> MEDVEIKPRGYQLRLVDHLTKSNGIVYLPTGSGKTFVAILVLKRFSQDFDKPIESGGKRALFMCNTVELARQQAMAVRRCTNFKVGFYVGEQGVDDWTRGMWSDEIKKNQVLVGTAQVFLDMVTQTYVALSSLSVVIIDECHHGTGHHPFREFMRLFTIANQTKLPRVVGLTGVLIKGNEITNVATKLKELEITYRGNIITVSDTKEMENVMLYATKPTEVMVSFPHQEQVLTVTRLISAEIEKFYVSLDLMNIGVQPIRRSKSLQCLRDPSKKSFVKQLFNDFLYQMKEYGIYAASIAIISLIVEFDIKRRQAETLSVKLMHRTALTLCEKIRHLLVQKLQDMTYDDDDDNVNTEEVIMNFSTPKVQRFLMSLKVSFADKDPKDICCLVFVERRYTCKCIYGLLLNYIQSTPELRNVLTPQFMVGRNNISPDFESVLERKWQKSAIQQFRDGNANLMICSSVLEEGIDVQACNHVFILDPVKTFNMYVQSKGRARTTEAKFVLFTADKEREKTIQQIYQYRKAHNDIAEYLKDRVLEKTEPELYEIKGHFQDDIDPFTNENGAVLLPNNALAILHRYCQTIPTDAFGFVIPWFHVLQEDERDRIFGVSAKGKHVISINMPVNCMLRDTIYSDPMDNVKTAKISAAFKACKVLYSLGELNERFVPKTLKERVASIADVHFEHWNKYGDSVTATVNKADKSKDRTYKTECPLEFYDALPRVGEICYAYEIFLEPQFESCEYTEHMYLNLQTPRNYAILLRNKLPRLA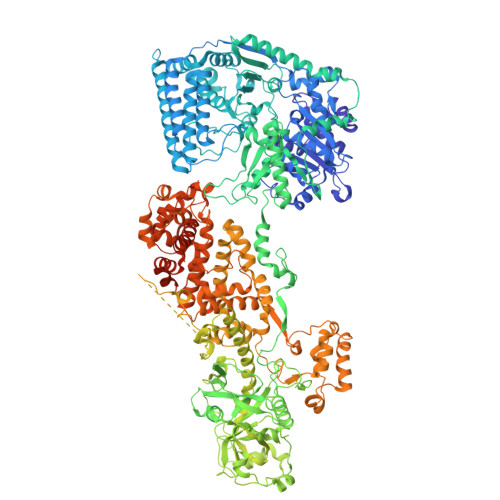EMPLFSNQGKLHVRVANAPLEVIIQNSEQLELLHQFHGMVFRDILKIWHPFFVLDRRSKENSYLVVPLILGAGEQKCFDWELMTNFRRLPQSHGSNVQQREQQPAPRPEDFEGKIVTQWYANYDKPMLVTKVHRELTPLSYMEKNQQDKTYYEFTMSKYGNRIGDVVHKDKFMIEVRDLTEQLTFYVHNRGKFNAKSKAKMKVILIPELCFNFNFPGDLWLKLIFLPSILNRMYFLLHAEALRKRFNTYLNLHLLPFNGTDYMPRPLEIDYSLKRNVDPLGNVIPTEDIEEPKSLLEPMPTKSIEASVANLEITEFENPWQKYMEPVDLSRNLLSTYPVELDYYYHFSVGNVCEMNEMDFEDKEYWAKNQFHMPTGNIYGNRTPAKTNANVPALMPSKPTVRGKVKPLLILQKTVSKEHITPAEQGEFLAAITASSAADVFDMERLEILGDSFLKLSATLYLASKYSDWNEGTLTEVKSKLVSNRNLLFCLIDADIPKTLNTIQFTPRYTWLPPGISLPHNVLALWRENPEFAKIIGPHNLRDLALGDEESLVKGNCSDINYNRFVEGCRANGQSFYAGADFSSEVNFCVGLVTIPNKVIADTLEALLGVIVKNYGLQHAFKMLEYFKICRADIDKPLTQLLNLELGGKKMRANVNTTEIDGFLINHYYLEKNLGYTFKDRRYLLQALTHPSYPTNRITGSYQELEFIGDAILDFLISAYIFENNTKMNPGALTDLRSALVNNTTLACICVRHRLHFFILAENAKLSEIISKFVNFQESQGHRVTNYVRILLEEADVQPTPLDLDDELDMTELPHANKCISQEAEKGVPPKGEFNMSTNVDVPKALGDVLEALIAAVYLDCRDLQRTWEVIFNLFEPELQEFTRKVPINHIRQLVEHKHAKPVFSSPIVEGETVMVSCQFTCMEKTIKVYGFGSNKDQAKLSAAKHALQQLSKCDA> HHHHHHSSGLVPRGSHMTPKDDEFYQQWQLKYPKLILREASSVSEELHKEVQEAFLTLHKHGCLFRDLVRIQGKDLLTPVSRILIGNPGCTYKYLNTRLFTVPWPVKGSNIKHTEAEIAAACETFLKLNDYLQIETIQALEELAAKEKANEDAVPLCMSADFPRVGMGSSYNGQDEVDIKSRAAYNVTLLNFMDPQKMPYLKEEPYFGMGKMAVSWHHDENLVDRSAVAVYSYSCEGPEEESEDDSHLEGRDPDIWHVGFKISWDIETPGLAIPLHQGDCYFMLDDLNATHQHCVLAGSQPRFSSTHRVAECSTGTLDYILQRCQLALQNVCDDVDNDDVSLKSFEPAVLKQGEEIHNEVEFEWLRQFWFQGNRYRKCTDWWCQPMAQLEALWKKMEGVTNAVLHEVKREGLPVEQRNEILTAILASLTARQNLRREWHARCQSRIARTLPADQKPE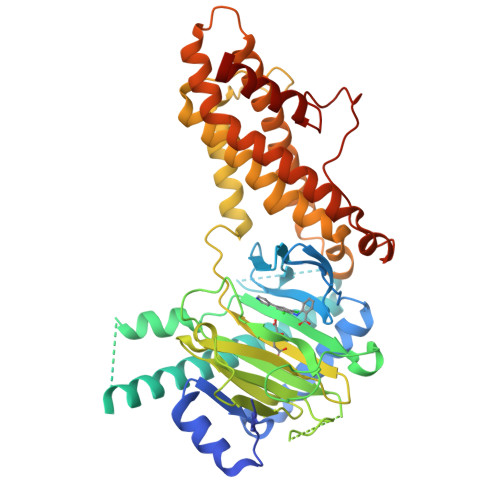CRPYWEKDDASMPLPFDLTDIVSELRGQLLEAKP> LEPEPWFFKNLSRKDAERQLLAPGNTHGSFLIRESESTAGSFSLSVRDFDQNQGEVVKHYKIRNLDNGGFYIS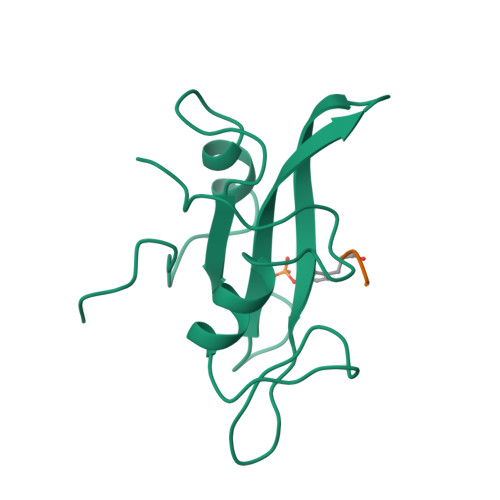PRITFPGLHELVRHYTNASDGLCTRLSRPCQT;> XYEEI>VFHKIRNEDLIFNESLGQGTFTKIFKGVRREVGDYGQLHETEVLL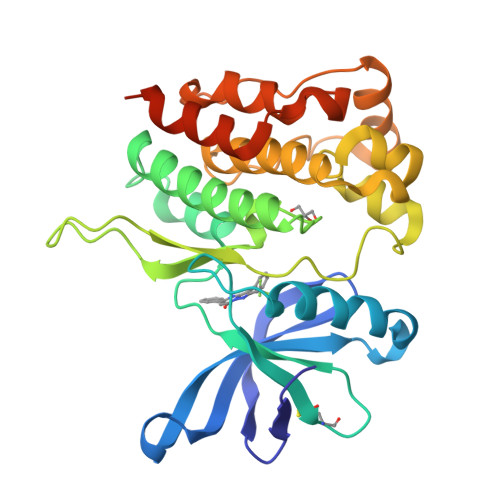KVLDKAHRNYSESFFEAASMMSKLSHKHLVLNYGVCVCGDENILVQEFVKFGSLDTYLKKNKNCINILWKLEVAKQLAAAMHFLEENTLIHGNVCAKNILLISEEDRKTGNPPFIKLSDPGISITVLPKDILQERIPWVPPECIENPKNLNLATDKWSFGTTLWEICSGGDKPLSALDSQRKLQFYEDRHQLPAPKAAELANLINNCMDYEPDHRPSFRAIIRDLNSLFTPDLVPRGSHHHHHH[2x]> PHEYEKDGAKIYVQSFATIRAEADLARFTPEEEVVVVRMIHAAGMVGLENHVRFAPGMAIAARAALEAGAPILCDARMVSEGIARARLPAKNEVICTLQDPRVPALAQEMGNTRSAAALELWRPKLEGAVVAIGNAPTALFHLLNMLEDPACPRPAAIIGCPV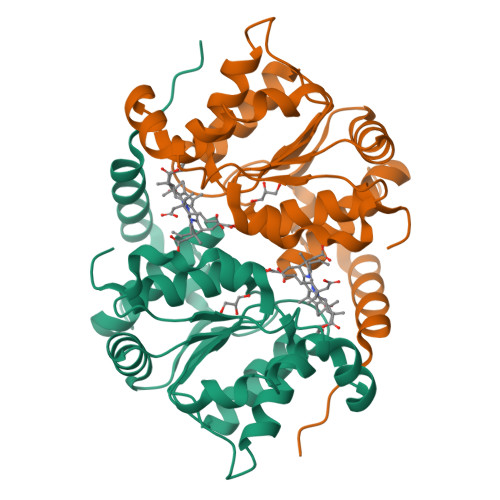GFIGAAESKAALAVANPVPWVIVEGRLGGSAITVAAVNALACRKE> MDSTGRAYDGASEFKSVLVTEGTSHYTPVEVYNILDELKTIKITSTIAEQSVVSRTPIPLSKIGLQDVKKLFDINVIKCGSSLRIVDEPQVTFIVSYAKDIYDKFMCIEHDSAYEPSLTMHRVRVIYSMLNDYCAKMISEVPYESSFVGELPVKSVTLNKLGDRNMDALAEHLLFEHDVVNAQRENRIFYQRKSAPAVPVIFGDDLEPAVRERANLYHRYSVPYHQIELALHALANDLLSIQYCHPTVVYNYLSSRAPNFLRLDDQVSLKLTSAGIGTLMPRPVVQLLDYDLVYMSPLALNNLASRLLRKISLHLVMQMVTAVQQDLGEVVSVSSNVTNPASACLVRMNVQGVQTLAVFIAQSMLNPNISYGMISGLTLDCFSNFIYGACLMLFQALIPPSALTARQRLDINNRFAYFLIKCHATQATTARLVANQVIYPVDAIDQWQSNGRDVLVAIYNNLLPGELVLTNLIQTYFRGNTAQQAAEILIPADQTSYGANETRALSAPYLFGAPINMLAPDARLSTYKRDLALPDRSPILITTVEGQNSISIENLRHKTGLIRAMYLNGFVTQPPAWIRNANSNTALLSRFLDATPNLLGIYEAILANTYANAVNVYCDSVYRADIPIEWKLHQSVDPQDLLFGVFGIVPQYQILNEAVPDFFAGGEDILILQLIRAVYDTLSNKLGRNPADIFHLEEVFKVIEEIVSVLVQQKIDVRKYFTESMRSGSFSKPRWDNFLRRPVAQRLPNLYSVIMTQADHVYNYMTQLTHIIPITDCFYIVKNSGFVDRGSTGPVIASSSVYENVLKVVHTIADFDAANALRLQRRRVDNTSYTDSLSDMFNGLRSISSSEFVRSVNGRSVFTEGRIDAIKVNMRAKFDLQFITEEGGYSKPPNVKKLMFSDFLSFLDSHKSDYRPPLLTVPITIGLNNLGETNSNTLRMRSEAIDEYFSSYVGAQILVPINVVDTRVYTEFS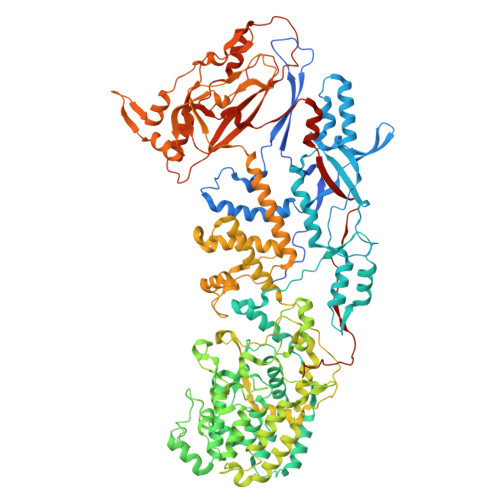ELRNFFTGDVVIRDDPFDVWDGVKATYIPIGVHGVRLDPNGDQPPL> DDAAIKRKLQSFNISNIVIKSSPISGIKTAVTDQGILYVSEDGKYLFEGKLYELTNNGPVDVAGKILVDKLNSYKDEMIVYPAKNEKHVVTVFMDITCHYCHLLHQQLKEYNDLGITVRYLAFPRAGMNNQTAKQMEAIWTAKDPVFALNEAEKGNLPKEVKTPNIVKKHYELGIQFGVRGTPSIVTSTGELIGGYLKPA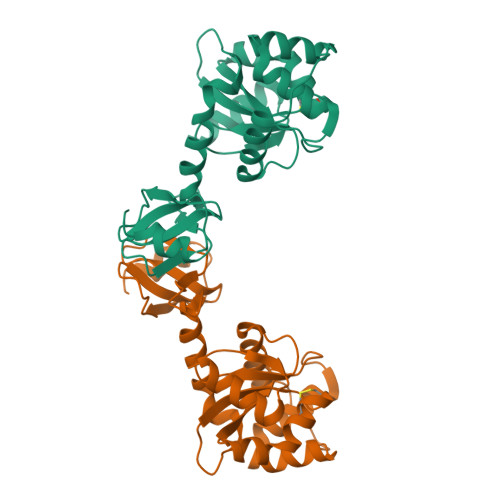DLLRALEETAQ> LSISPIFQGGSYQLNNKSIDISSLLLDKLSGESQTVVMKFKADKPNSLQALFGLSNSKAGFKNNYFSIFMRDSGEIGVEIRDAQKGINYLFSRPASLWGKHKGQAVENTLVFVS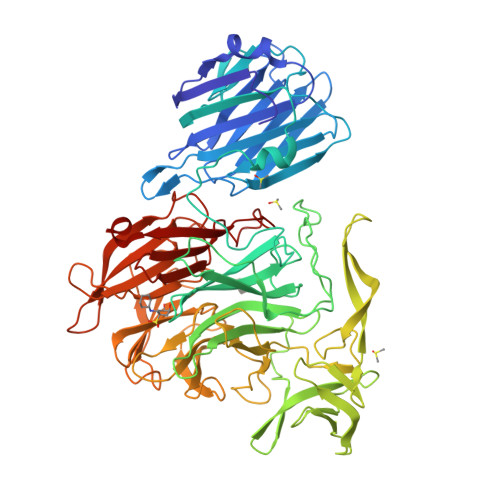DSKDKTYTMYVNGIEVFSETVDTFLPISNINGIDKATLGAVNREGKEHYLAKGSIDEISLFNKAISDQEVSTIPLSNPFQLIFQSGDSTQANYFRIPTLYTLSSGRVLSSIDARYGGTHDSKSKINIATSYSDDNGKTWSEPIFAMKFNDYEEQLVYWPRDNKLKNSQISGSASFIDSSIVEDKKSGKTILLADVMPAGIGNNNANKADSGFKEINGHYYLKLKKNGDNDFRYTVRENGVVYNETTNKPTNYTINDKYEVLEGGKSLTVEQYSVDFDSGSLRERHNGKQVPMNVFYKDSLFKVTPTNYIAMTTSQNRGESWEQFKLLPPFLGEKHNGTYLCPGQGLALKSSNRLIFATYTSGELTYLISDDSGQTWKKSSASIPFKNATAEAQMVELRDGVIRTFFRTTTGKIAYMTSRDSGETWSKVSYIDGIQQTSYGTQVSAIKYSQLIDGKEAVILSTPNSRSGRKGGQLVVGLVNKEDDSIDWKYHYGIDLPSYGYAYSAITELPNHHIGVLFEKYDSWSRNELHLSNVVQYIDLEINDLT>MIPDVSQALAWLEKHPQALKGIQRGLERETLRVNADGTLATTGHPEALGSALTHKWITTDFAEALLEFITPVDGDIEHMLTFMRDLHRYTARNMGDERMWPLSMPSYIAEGQDIELAQYGTSNTGRFKTLYREGLKNRYGALMQTISGVHYNFSLPMAFWQAKSGDISGADAKEKISAGYFRVIRNYYRFGWVIPYLFGASPAISSSFLQGKPTSLPFEKTESGMYYLPYATSLRLSDLGYTNKSQSNLGITFNDLYEYVAGLKQAIKTPSEEYAKIGIEKDGKRLQINSNVLQIENELYAPIRPKRVTRSGESPSDALLRGGIEYIEVRSLDINPFSPIGVDEQQVRFLDLFMVW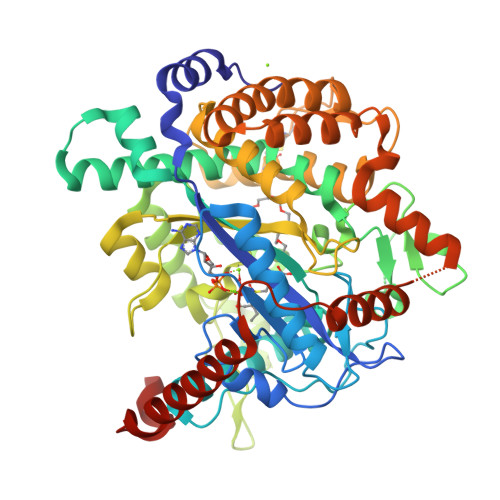CALADAPEMSSSELACTRVNWNRVILEGRKPGLTLGIGCETAQFPLPQVGKDLFRDLKRVAQTLDSINGGEAYQKVCDELVACFDNPDLTFSARILRSMIDTGIGGTGKAFAEAYRNLLREEPLEILREEDFVAEREASERRQQEMEAADTEPFAVWLEKHA[2x]>[2x]GPLGSMVTEQEVDAIGQTLVDPKQPLQARFRALFTLRGLGGPGAIAWISQAFDDDSALLKHELAYCLGQMQDARAIPMLVDVLQDTRQEPMVRHEAGEALGAIGDPEVLEILKQYSSDPVIEVAETCQLAVRRLEWLQQHGGEPAAGPYLSVDPAPPAEERDVGRLREALLDESRPLFERYRAMFALRNAGGEEAALALAEGLHCGSALFR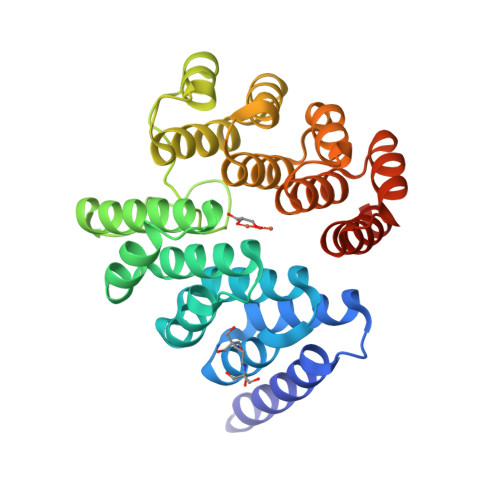HEVGYVLGQLQHEAAVPQLAAALARCTENPMVRHECAEALGAIARPACLAALQAHADDPERVVRESCEVALDMYEHETGRAFQ> MLNGPSIIISLFFCFVSGAYACCKCDCQSGWEWFGGSCYLFDETERGWEDSKTFCESQNAALVTVESSEEDDFIRGVISAQSAFHYYWIGGSWDAEHSEYRWIDGSSISFNGW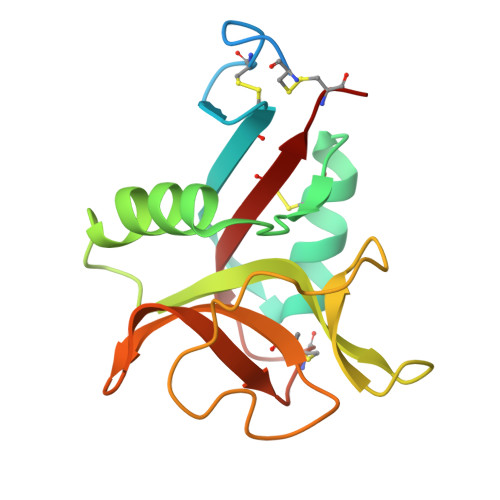GPNRPDADEGCMDYLNYKEIVWQWNDHQDCVNTKGPSICETDCSE>[4x]SHME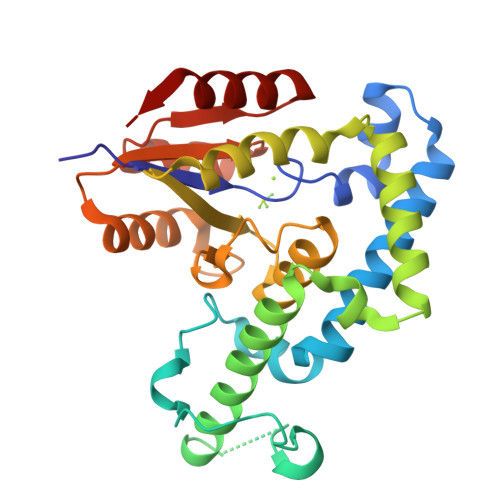RVFVWDLDETIIIFHSLLTGTFASRYGKDTTTSVRIGLMMEEMIFNLADTHLFFNDLEDCDQIHVDDVSSDDNGQDLSTYNFSADGFHSSAPAANLCLGSGVHGGVDWMRKLAFRYRRVKEMYNTYKNNVGGLIGTPKRETWLQLRAELEALTDLWLTHSLKALNLINSRPNCVNVLVTTTQLIPALAKVLLYGLGSVFPIENIYSATKTGKESCFERIMQRFGRKAVYVVIGDGVEEEQGAKKHNMPFWRISCHADLEALRHALELEYL>MTPLGPASSLPQSFLLKCLEQVRKIQGDGAALQEKLCATYKLCHPEELVLLGHSLGIPWAPLSSCPSQALQLAGCLSQLHSGLFLYQGLLQALEGISPELGPTLDTLQLDVADFATTIWQQMEELGMAPALQPTQGAMPAFASAFQRRAGGVLVASHLQSFLEVSYRVLRHLAQP[4x];>[4x]AGYPPASPSNLSCLMHLTTNSLVCQWEPGPETHLPTSFILKSFRSRADCQYQGDTIPDCVAKKRQNNCSIPRKNLLLYQYMAIWVQAENMLGSSESPKLCLDPMDVVKLEPPMLQALDIGPDVVSHQPGCLWLSWKPWKPSEYMEQECELRYQPQLKGANWTLVFHLPSSKDQ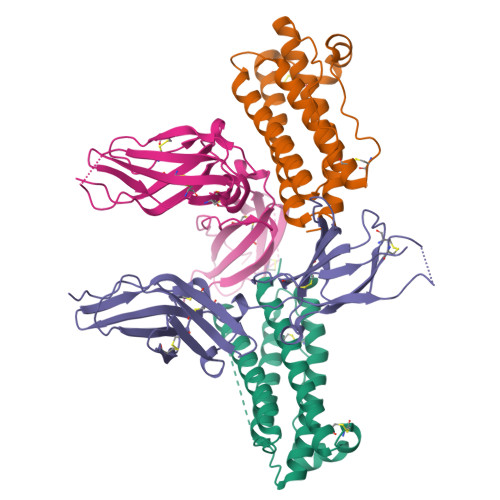FELCGLHQAPVYTLQMRCIRSSLPGFWSPWSPGLQLRPTMKA>ALTNAQILAVIDSWEETVGQFPVITHHVPLGGGLQGTLHCYEIPLAAPYGVGFAKNGPTRWQYKRTINQVVHRWGSHTVPFLLEPDNINGKTCTASALCHNTRCHNPLHLCWESLDDNKGRNWCPGPNGGCVHAVVCLRQGPLYGPGATVAGPQQRGSHFVV[2x]

I-PpoI is a well-characterized intron-encoded homing endonuclease member of the physarum polycephalum slimemold. A large subfamily of one-metal-ion-dependent nucleases consist of histidine-metal (His-Me) nucleases that perform critical tasks in biological pathways such as apoptosis, extracellular defense, intracellular immunity (CRISPR–Cas9), and intron homing (homing endonuclease). Surrounded by two beta sheets and an alpha helix, the His-Me nucleases active sites all contain a single metal ion, a histidine, and an asparagine. The asparagine residue helps to stabilize metal ion binding whereas the strictly conserved histidine is suggested to deprotonate a nearby water for nucleophilic attack toward the scissile phosphate.

Because His98 has been proposed to primarily activate the nucleophilic water, we first mutated His98 to alanine. To confirm divalent metal ion binding, the H98A I-PpoI crystals were soaked for 1800s in 500 µM Mn2+, the same concentration used to initiate DNA hydrolysis by WT I-PpoI. However, to our surprise, the metal ion-binding site was devoid of any anomalous signal. Increasing the Mn2+ concentration to 1 mM still did not produce anomalous density at the Me2+-binding site. (D) Structure of H98A I-PpoI active site after 1 mM Mn2+ soaking for 1800s. The results indicate that metal ion binding can be altered by perturbing His98 and possibly water deprotonation, even though the metal ion-binding site and His98 exist 7 Å apart without direct interaction. Moreover, the metal ion was not observed in crystallo when His98 was removed. Without a proper proton acceptor, the metal ion may be prone for dissociation without the reaction proceeding, and thus stable Mg2+ binding was not observed in crystallo without His98. Our results indicate that perturbing the deprotonation pathway not only affects nucleophilic attack but also metal binding, suggesting that I-PpoI catalyzes DNA catalysis via a concerted mechanism.The Schlafen family belongs to the interferon-stimulated genes and its members are involved in cell cycle regulation, T cell quiescence, inhibition of viral replication, DNA-repair and tRNA processing. Here, we present the cryo-EM structure of full-length human Schlafen 5 (SLFN5) and the high-resolution crystal structure of the highly conserved N-terminal core domain. SLFN5 binds tRNA as well as single- and double-stranded DNA, suggesting a potential role in transcriptional regulation. The N-terminal Slfn core domain (residues 1–336) is followed by a linker domain (residues 337–552) and a C-terminal helicase/ ATPase domain (residues 553–891).

To gain high resolution structural insights into human SLFN5, we crystallized the SLFN5 core domain (SLFN51–336). SLFN51–336 crystallized in the space groups P3221 and P21, diffracting to 3.2 and 1.8 Å, respectively. The structure was determined by SAD using the intrinsically bound zinc ion and was refined to a resolution of 1.8 Å. The crystal structure, at a resolution of 1.8 Å, revealed a highly conserved zinc finger motif. The SLFN51- 336 structure depicts a horseshoe-like shape with a mixed α/β topology consisting of 10 α-helices and 14 β-sheets. The approximate dimensions are 63 × 40 × 25 Å with the inner tunnel measuring 18 Å. The SLFN51–336 structure comprises a zinc finger motif with the calculated anomalous map confirming the presence of a zinc ion. The zinc ion is coordinated by a histidine and three cysteine residues (H266, C268, C302, C303) that are highly conserved throughout the entire Schlafen protein family. The electron density for residues 145–168 could not be traced, indicating that this region consists of a flexible loop. When comparing these residues in the crystal structures of SLFN51–336 and rSlfn13 to the active sites of other ATPases, no explicit structural similarity is evident.

>MSLRIDVDTNFPECVVDAGKVTLGTQQRQEMDPRLREKQNEIILRAVCALLNSGGGIIKAEIENKGYNYERHGVGLDVPPIFRSHLDKMQKENHFLIFVKSWNTEAGVPLATLCSNLYHRERTSTDVMDSQEALAFLKCRTQTPTNINVSNSLGPQAAQGSVQYEGNINVSAAALFDRKRLQYLEKLNLPESTHVEFVMFSTDVSHCVKDRLPKCVSAFANTEGGYVFFGVHDETCQVIGCEKEKIDLTSLRASIDGCIKKLPVHHFCTQRPEIKYVLNFLEVHDKGALRGYVCAIKVEKFCCAVFAKVPSSWQVKDNRVRQLPTREWTAWMMEADHHHHHH[2x]>MTDVQCEPALAGRKPKWADADIAELVDERTGRLDPRIYTDEALYEQELERIFGRSWLLMGHETQIPKAGDFMTNYMGEDPVMVVRQKNGEIRVFLNQCRHRGMRICRADGGNAKSFTCSYHGWAYDTGGNLVSVPFEEQAFPGLRKEDWGPLQARVETYKGLIFANWDADAPDLDTYLGEAKFYMDHMLDRTEAGTEAIPGIQKWVIPCNWKFAAEQFCSDMYHAGTTSHLSGILAGLPDGVDLSELAPPTEGIQYRATWGGHGSGFYIGDPNLLLAIMGPKVTEYWTQGPAAEKASERLGSTERGQQLMAQHMTIFPTCSFLPGINTIRAWHPRGPNEIEVWAFTVVDADAPEEMKEEYRQQTLRTFSAGGVFEQDDGENWVEIQQVLRGHKARSRPFNAEMGLGQTDSDNPDYPGTISYVYSEEAARGLYTQWVRMMTSPDWAALDATRPAVSESTHT[3x];>[3x]MIDAESPTTAFRTKPAPVDPSLQHEIEQFYYWEAKLLNDRRF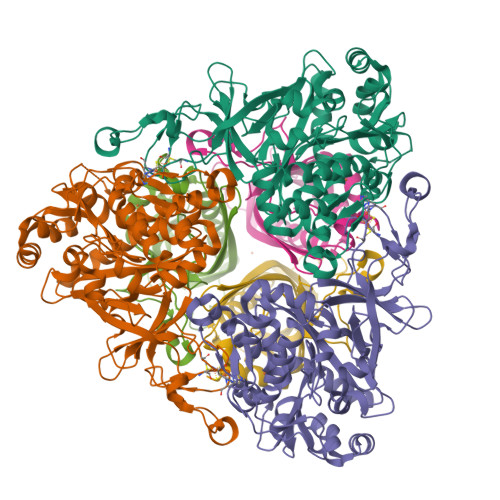QEWFDLLAEDIHYFMPIRTTRIMRETAQEYSGAREYAHFDDNAQMMRGRLRKITSDVSWSENPASRTRHVISNVMIVDGEKPGEYHVSSVFIVYRNRLERQLDIFAGERKDILRRTGSEAGFELAKRTILIDQSTILSNNLSFFF>[4x]FPQLPPAPDDYP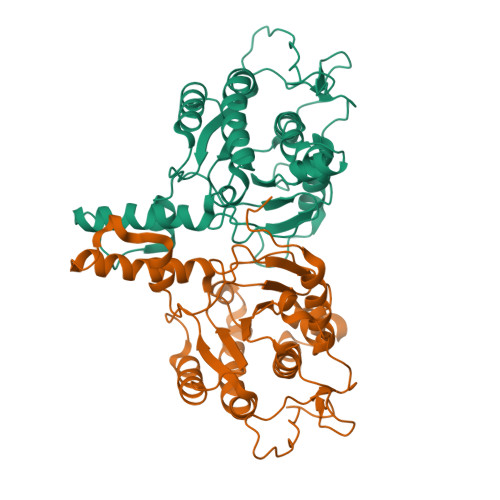TFPDTSTWPVVFPELPAAPYGGPCRPPQHTSKAAAPRIPADRLPNHVAIVMDGNGRWATQRGLARTEGHKMGEAVVIDIACGAIELGIKWLSLYAFSTENWKRSPEEVRFLMGFNRDVVRRRRDTLKKLGVRIRWVGSRPRLWRSVINELAVAEEMTKSNDVITINYCVNYGGRTEITEATREIAREVAAGRLNPERITESTIARHLQRPDIPDVDLFLRTSGEQRSSNFMLWQAAYAEYIFQDKLWPDYDRRDLWAACEEYASRTRRFGSA SPECTINOMYCIN | 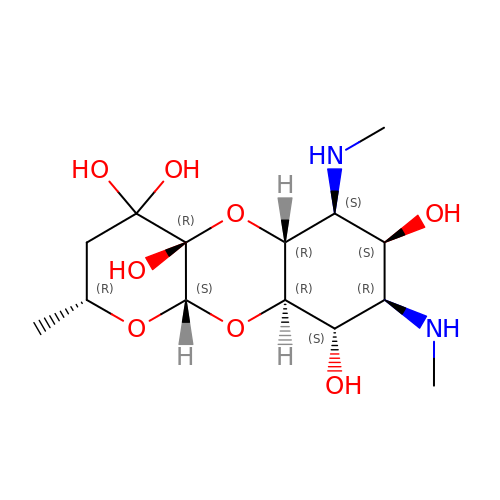C14 H26 N2 O8 | JEBSYFSDBYNEEU-GOZOPVAMSA-N> MAPTPKYTFTERAA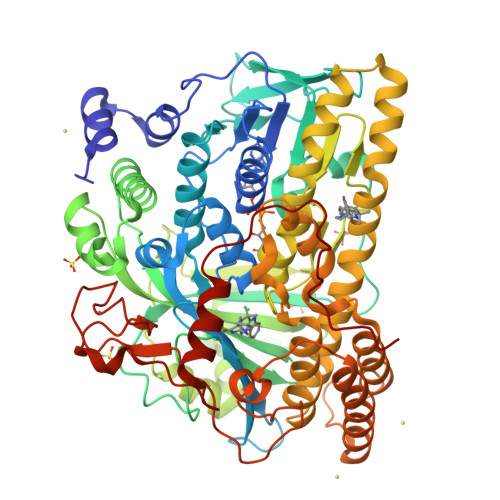AGNLSDAEILNSNNPTGSELPDESDVVVGGAGIHGLIYALHASKYKPNNLKISVIEKNTRPGYKIGESTLPIFYTWCKLHGISAAYLLRLFGLKDGLCFYFLDRENQGQYTDFCSVGAPGLVLASLQIERPMSELLFTILAQRNGVNVYHGREVDFKSTVVQGGGQGNKIAVSRGKYDSTPKTIDSALFVDATGRFRQFCSKKAPRHRFDGWNCNAFWGYFTAPKDESKIPFDLYEGDFTNHLCFPEGWVWVIRLPSWEGSPIANLMDMVTYILECADAGVPGDELPSSEELARMFGLKFQWVTSIGFAVRNDVKYPEDLSAYGTREAEQKFNYFVQKYELLQQFMSNFELIENLYGPGTTWFIRKTLAYQSPVVSGPGWLAIGDACGFTNPLYSPGINVGMSTSTWAAQLSHPIVEIGKSAPADAAESSIRKLLVPYDDYCKSLVPALEQMNRFNYVCYRDTRLGPQVACLWQFFAGIERYLSDVNIETFAHYAIKWVWGAMVPEYQQVAQKCIEHIETVPLDERLPDAMVDELLAFSNRIKSAAVAADDFSLRWDAILRSFDRSLNFVEGKTSRDIYTRQCSGCGAWLQLRPDWKKCHSCGLLGTEPQTAVTFDPPLTAEEEALLYAAWNTAPKYDPSKELKLPTPTRPAA> GPEEIRPKE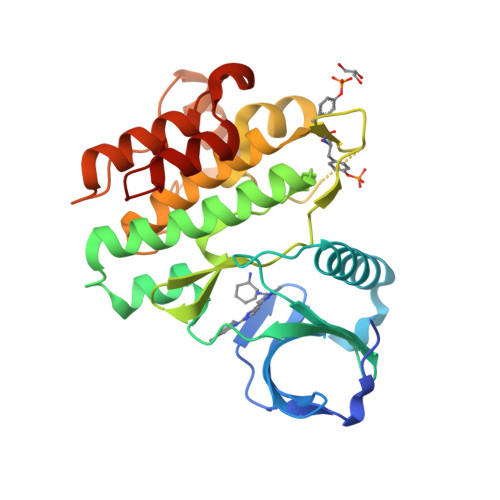VYLDRKLLTLEDKELGSGNFGTVKKGYYQMKKVVKTVAVKILKNEANDPALKDELLAEANVMQQLDNPYIVRMIGICEAESWMLVMEMAELGPLNKYLQQNRHVKDKNIIELVHQVSMGMKYLEESNFVHRDLAARNVLLVTQHYAKISDFGLSKALRADENYYKAQTHGKWPVKWYAPECINYYKFSSKSDVWSFGVLMWEAFSYGQKPYRGMKGSEVTAMLEKGERMGCPAGCPREMYDLMNLCWTYDVENRPGFAAVELRLRNYYYDVVN>MSNLPVEPEFEQAYKELASTLENSTLFQKNPEYRKALAVVSVPERVIQFRVVWENDKGEVQVNRGFRVQFNSALGPYKGGLRFHPSVNLSILKFLGFEQIFKNALTGLNMGGGKGGSDFDPKGKSDSEIRRFCVAFMTELCRHIGADTDVPAGDIGVTGREIGYLFGQYRKLRNSWEGVLTGKGGSWGGSLIRPEATGYGVVYYVEHMIAHATNGAESFAGKRVAISGSGNVAQYAALKVIELGGRVVSLSDSQGSLIVKDTAKDSFTPAEIDAIAALKVDRKQIAELVTDAAFADKFTYLPGQRPWVHVGAVDVALPSATQNEVSGEEAQALIAAGCKFIAEGSNMGCTQAAIDAFEAHREANKGAAAIWYAPGKAANAGGVAVSGLEMAQNSARLSWTAEEVDARLKDIMKSCFQNGLDTAKEYAT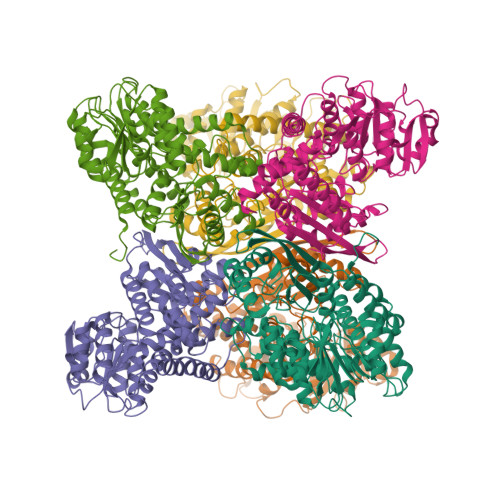PADGILPSLVTGSNIAGFTKVAAAMKDQGDWW[6x]> MGDKKGKKKGGGEEDESTLQLSRQYKKKCELNGINPSKLFKEKLDFAVEEDENIEKIHLWEELGPVGVRSIMDSLTEIPYLHTKSIRLWKVKAQDEGTRTICNYMEKSKTIEYLDLMDNQVGSLGCEFLGRVLHPQIEIPLLKLKLDHNEFGTEGLMQLAAGLCMNSVLEKLSLNYCAITAEGSKYIQQILSFVNTNLKKLKMKGNLL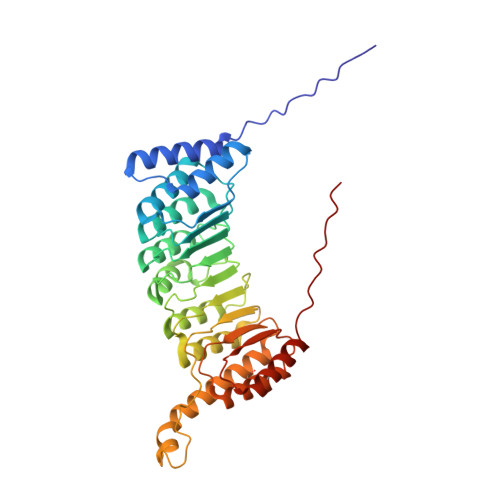KNEGVHQLFRAFKVNKTLEKVDLSDNQFDTTLGDDQDPEANPNFFETNKDAIEHNKQIIENICEVLKAADTLLYYDFRFNNISKTDAKAIIDCLEANKNIYYMELSEHIPKDLIERKKGLMKKRKPKKKKKKKAKKK> GSHMASMKKKGSVVIVG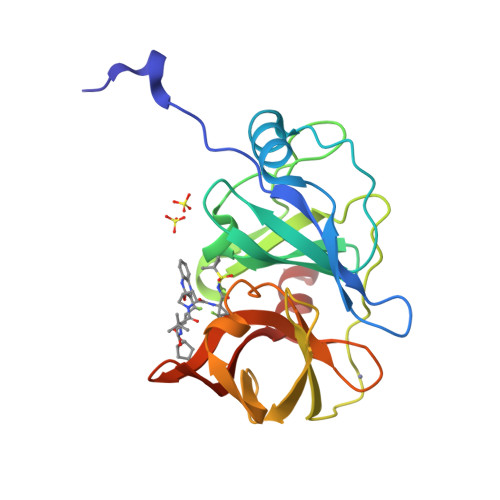RINLSGDTAYAQQTRGEEGCQETSQTGRDKNQVEGEVQIVSTATQTFLATSINGVLWTVYHGAGTRTIASPKGPVTQMYTNVDKDLVGWQAPQGSRSLTPCTCGSSDLYLVTRHADVIPVRRRGDSRGSLLSPRPISYLKGSSGGPLLCPAGHAVGIFRAAVCTRGVAKAVEFIPVESLETTMRA> SVEPYSDAAFTQAQASGAPVLVDVYADWCPVCKRQERELTPLFAQPAQRDLR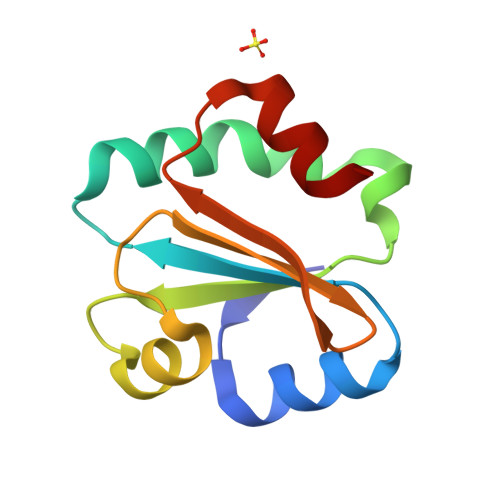VFKVNFDTQKAALQQFRVSQQSTLILYRNGQEVRRSIGETSPSALSDFLTR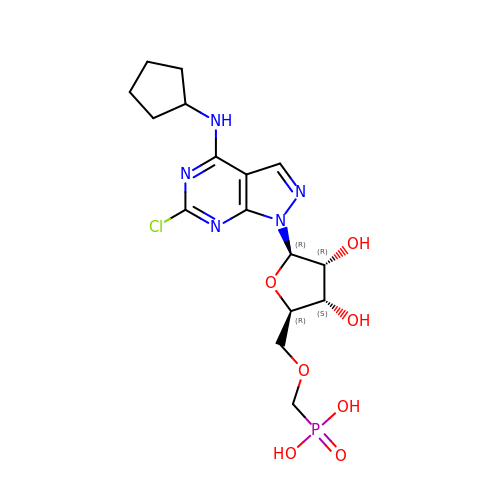[(2~{R},3~{S},4~{R},5~{R})-5-[6-chloranyl-4-(cyclopentylamino)pyrazolo[3,4-d]pyrimidin-1-yl]-3,4-bis(oxidanyl)oxolan-2-yl]methoxymethylphosphonic acid | C16 H23 Cl N5 O7 P | IVHVIBKVJIZKOC-RTWAVKEYSA-N> GSHMGEGVQLTAAQELMIQQLVAAQLQCNKRSFSDQPKVTPWPLGADPASGSASQQRFAHFTELAIISVQEIVDFAKQVPGFLQLGREDQIALLKAS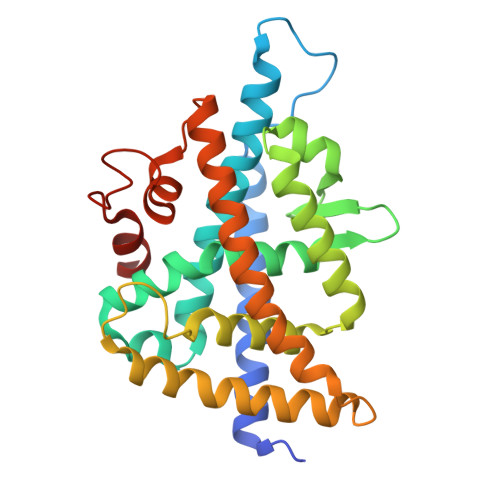TIEIMLLETARRYNHETECITFLKDFTYSKDDFHRAGLQVEFINPIFEFSRAMRRLGLDDAEYALLIAINIFSADRPNVQEPGRVEALQQPYVEALLSYTRIKRPQDQLRFPRMLMKLVSLRTLSSVHSEQVFALRLQDKKLPPLLSEIWDVHEGSGSGSHKILHRLLQDSSS>[2x]MTKVLVLGGRFGAL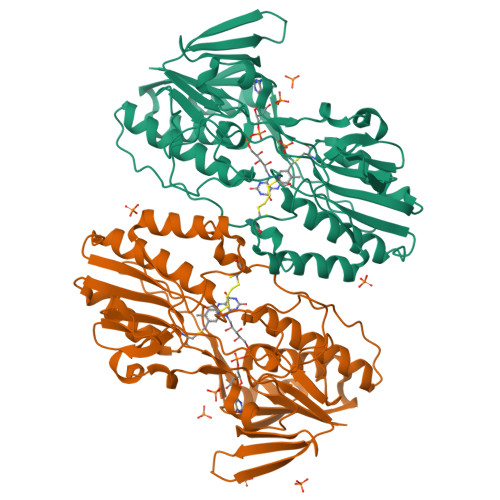TAAYTLKRLVGSKADVKVINKSRFSYFRPALPHVAIGVRDVDELKVDLSEALPEKGIQFQEGTVEKIDAKSSMVYYTKPDGSMAEEEYDYVIVGIGAHLATELVKGWDKYGYSVCEPEFATKLREKLESFQGGNIAIGSGPFYQGHNPKPKVPENFVPNADSACEGPVFEMSLMLHGYFKKKGMLDKVHVTVFSPGEYLSDLSPNSRKAVASIYNQLGIKLVHNFKIKEIREHEIVDEKGNTIPADITILLPPYTGNPALKNSTPDLVDDGGFIPTDLNMVSIKYDNVYAVGDANSMTVPKLGYLAVMTGRIAAQHLANRLGVPTKVDKYYPTIVCVADNPYEGYAVSVKDDTWYGGTVSIADPAAVNHLKKELFTKYYMWTKGDMALEKFLASW>GPSRATMDTESTYSGYSYYSSHSKKSHRQGERTRERHKSPRNKDGRGSEKSVTIQPPTGEPLLGNDSTRTEEVQDDNWGETTTAITGTSEHSISQEDIARISKDMEDSVGLDCKRYLGLTVASFLGLLVFLTPIAFILLPPILWRDELEPCGTICEGLFISMAFKLLILLIGTWALFFRKRRADMPRVFVFRALLLVLIFLFVVSYWLFYGVRILDSRDRNYQGIVQYAVSLVDALLFIHYLAIVLLELRQLQPMFTLQVVRSTDGESRFYSLGHLSIQRAALVVLENYYKDFTIYNPNLLTASKFRAAKHMAGLKVYNVDGPSNNATGQSRAMIAAAARRRDSSHNELYYEEAEHERRVKKRKARL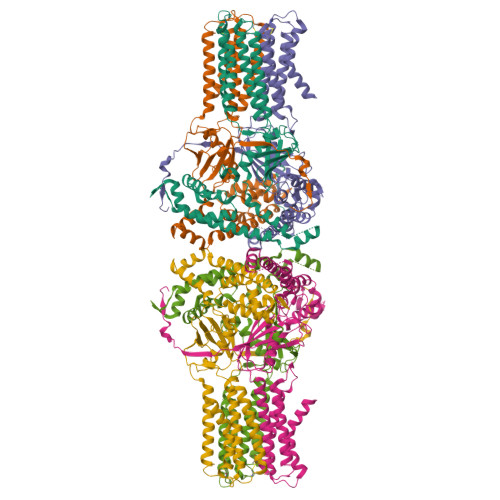VVAVEEAFIHIQRLQAEEQQKAPGEVMDPREAAQAIFPSMARALQKYLRITRQQNYHSMESILQHLAFCITNGMTPKAFLERYLSAGPTLQYDKDRWLSTQWRLVSDEAVTNGLRDGIVFVLKCLDFSLVVNVKKIPFIILSEEFIDPKSHKFVLRLQSETSV[6x]> MGSSHHHH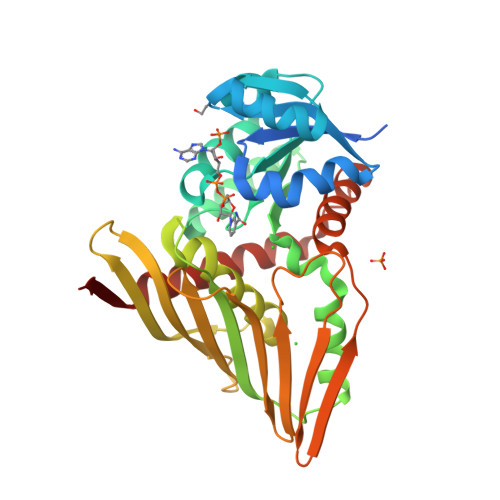HHENLYFQGHMENPANANPIRVGVIGCADIAWRRALPALEAEPLTEVTAIASRRWDRAKRFTERFGGEPVEGYPALLERDDVDAVYVPLPAVLHAEWIDRALRAGKHVLAEKPLTTDRPQAERLFAVARERGLLLMENFMFLHHPQHRQVADMLDEGVIGEIRSFAASFTIPPKPQGDIRYQADVGGGALLDIGVYPIRAAGLFLGADLEFVGAVLRHERDRDVVVGGNALLTTRQGVTAQLTFGMEHAYTNNYEFRGSTGRLWMNRVFTPPATYQPVVHIERQDHAEQFVLPAHDQFAKSIRAFAQAVLSGEHPREWSEDSLRQASLVDAVRTGARDIYFP> ICNGSLYPEPTLVPTPPPELPTDCGGPFELWEPNTTFSSTNFPNSYPNLAFCVWILNAQKGKNIQLHFQEFDLANINDVVEIRDGEEADSLLLAVYTGPGPVKDVFSTTNRMTVLLITNDVLARGGFKANFTTGYHLGIPEPCKADHFQCKNGECVPLVNLCDGHLHCEDGSDEADCVRFFNGTTNNNGLVRFRIQSIWHTACAENWTTQISNDVCQLLGLGSGNSSKPIFPTDGGPFVKLNTAPDGHLILTPSQQCLQDSLIRLQCNHKSCGKKLAAQDI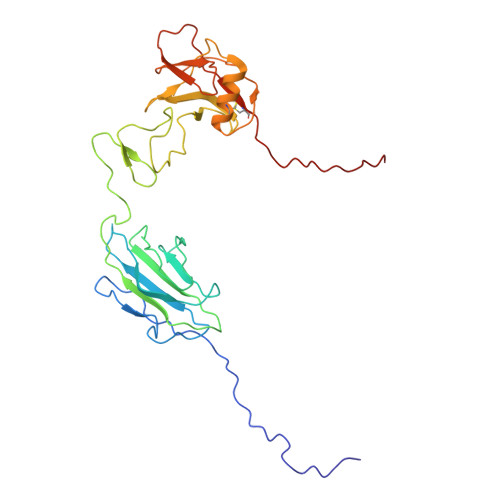TPK>[2x]PREYEFAEKILFTEEEIRTRIKEVAKRIADDYKGKGLRPYVNPLVLISVLKGSFMFTADLCRALCDFNVPVRMEFICVSSYGEGLTSSGQVRML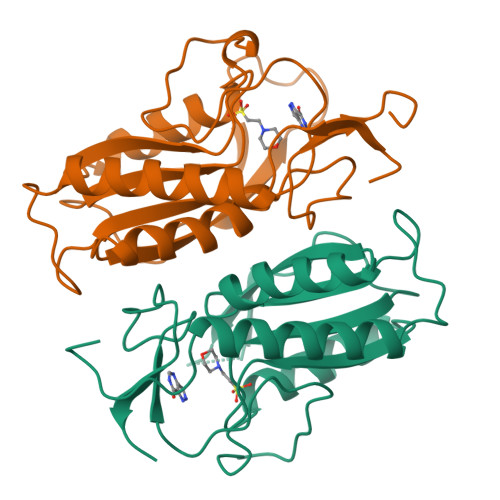LDTRHSIEGHHVLIVEDIVDTALTLNYLYHMYFTRRPASLKTVVLLDKREGRRVPFSADYVVANIPNAFVIGYGLDYDDTYRELRDIVVLRPEVYAEREAARQKKQRAIGSADTDRDAKREFHSKY>MQLTPTFYDNSCPNVSNIVRDTIVNELRSDPRIAASILRLHFHDCFVNGCDA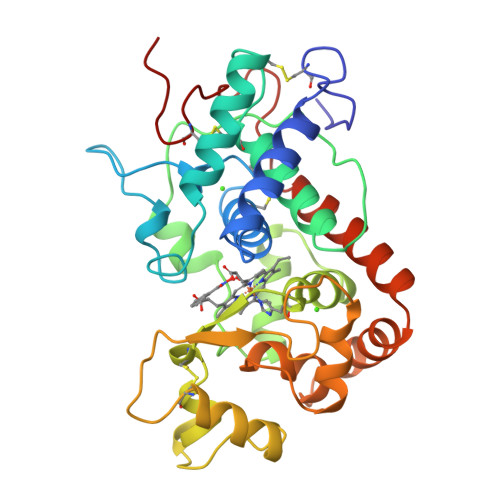SILLDNTTSFRTEKDAFGNANSARGFPVIDRMKAAVESACPRTVSCADLLTIAAQQSVTLAGGPSWRVPLGRRDSLQAFLDLANANLPAPFFTLPQLKDSFRNVGLNRSSDLVALSGGHTFGKNQCRFIMDRLYNFSNTGLPDPTLNTTYLQTLRGLCPLNGNLSALVDFDLRTPTIFDNKYYVNLEEQKGLIQSDQELFSSPNATDTIPLVRSFANSTQTFFNAFVEAMDRMGNITPLTGTQGQIRLNCRVVNSN[2x]> MAFGINYMGRVSTSANNDTQKVWIYNGTATGSNETVATIAASGYFNAFMVNVALGKGPLGVGDLIIINGNDASAFYTVQTITPNVTVSVFAASGVVGTSNIQDGAVTANKLATDSVTTVKILDDNVTSDKIAASVLKYVAVPLTAANIIAMNGAPVQVLAAGGANTVHLVEHACLMM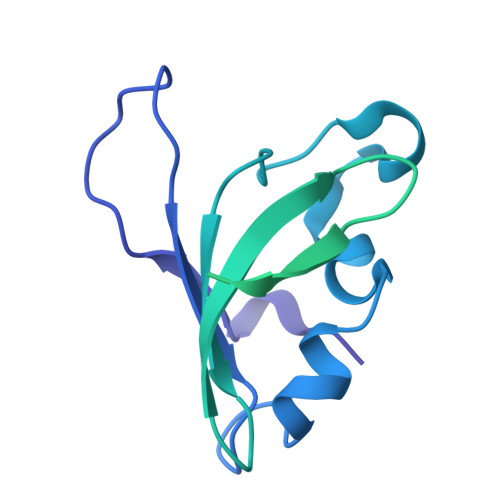TYGTTQFTGGGAIGLQYGNTAALAGEAASSTIAAANVQGAASTMDMVEGALSSGAFTAVANLGLFISNNTAAFAAGDSDFVLHLWYRTVPTV> MEKSFVITDPRLPDNPIIFASDGFLELTEYSREEILGRNGRFLQGPETDQATVQKIQDAIRDQREITVQLINYTKSGKKFWNLLHLQPMRDQKGELQYFIGVQLDGEFIP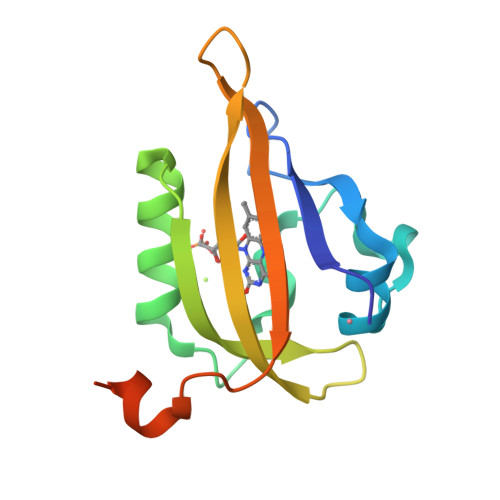NPLLGLDSTRTGHHHHHH>[2x]MDQKPQPAKTHATEVTVLEGKTMGTFWRASIPGIDAKRSAELKEKIQTQLDADDQLLSTNKKDSALMRFNDSQSLSPWPVSEAMADIVTTSLRIGAKTDGAMDITVGPLVNLWGFGPEQQPVQIPSQEQIDAMKAKTGLQHLTVINQSHQQYLQKDLPDLYVDLSTVGEGY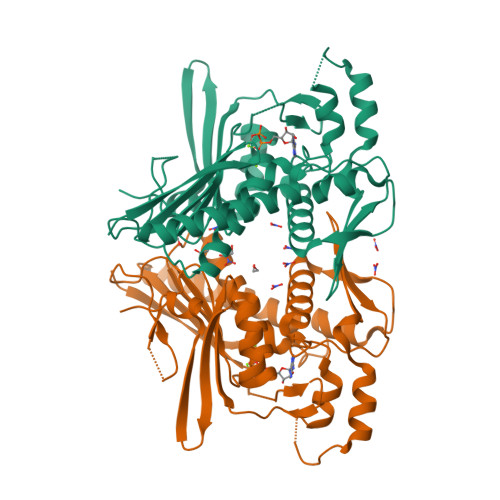AADHLARLMEQEGISRYLVSVGGALNSRGMNGEGLPWRVAIQKPTDKENAVQAVVDINGHGISTSGSYRNYYELDGKRLSHVIDPQTGRPIEHNLVSVTVIAPTALEADAWDTGLMVLGPEKAKEVVRREGLAVYMITKEGDSFKTWMSPQFKSFLVSEKNLEHHHHHH> PS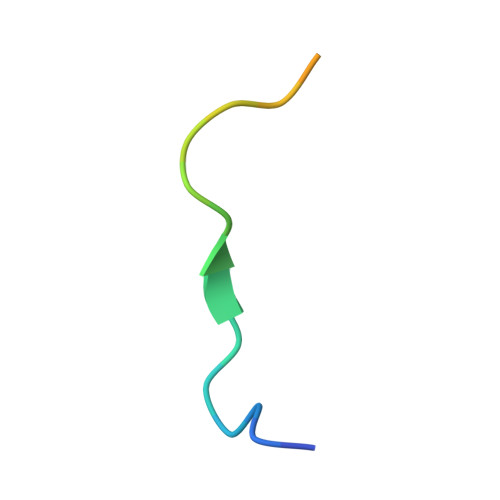CPKPVQDTQPPESPVENSE>MRGSHHHHHHGSLSSSPSEILQELGKGSTHPQPGVSPPAAPAAPGPKDGPGETDAFGNSEGKELVASGENKIKQGLLPSLEDLLFYTIAEGQEKIPVHKFITALKSTGLRTSDPRLKECMDMLRLTLQTTSDGVMLDKDLFKKCVQSNIVLLTQAFRRKFVIPDFMSFTSHIDELYESAKKQSGGKVADYIPQLAKFSPDLWGVSVCTVDGQRHSTGDTKVPFCLQSCVKPLKYAIAVNDLGTEYVHRYVGKEPSGLRFNKLFLNEDDKPHNPMVNAGAIVVTSLIKQGVNNAEKFDYVMQFLNKMAGNEYVGFSNATFQSERESGDRNFAIGYYLKEKKCFPEGTDMVGILDFYFQLCSIEVTCESASVMAATLANGGFCPITGERVLSPEAVRNTLSLMHSCGMYDFSGQFAFHVGLP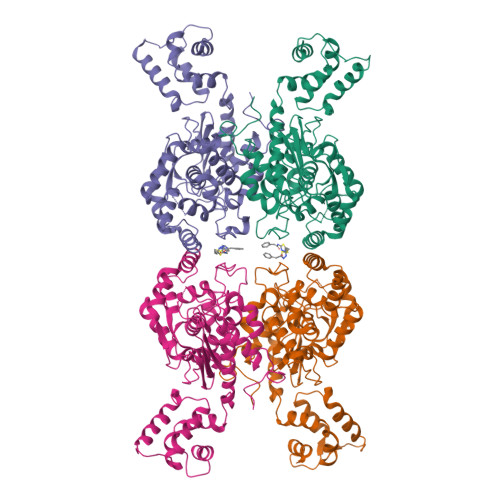AKSGVAGGILLVVPNVMGMMCWSPPLDKMGNSVKGIHFCHDLVSLCNFHNYDNLRHFAKKLDPRREGGDQR[4x]The reabsorption process of urate in the kidney by the urate transporter URAT1 plays a pivotal role in controlling serum urate levels. URAT1 (SLC22A12) is a member of the SLC22 major facilitator superfamily transporters. The cryo-EM structures show that hURAT1 has the common architecture of SLC22 family transporters, which is formed by the N-terminal domain (NTD) with an extracellular protrusion and the C-terminal domain (CTD). Structural comparison between different conformations of hURAT1 reveals the rocker-switch-like mechanism for urate transport.

In the presence of substrate urate, hURAT1 predominantly adopts the outward-facing conformation, in which regions of the NTD and CTD in the inner leaflet of the plasma membrane bind to each other to seal the intracellular gate. Urate binds in the center of the transmembrane domain of hURAT1. The three protrusions on the electron density match the three oxygens on urate, unambiguously defining the binding pose of urate. The xanthine core of urate is wrapped by a hydrophobic cage consisting of five phenylalanines, including F241 of the NTD and F360, F364, F365, and F449 of the CTD. In addition to the binding by these five phenylalanines, the negatively charged 2’-oxygen of urate (pKa ~5.4)20 is coordinated by R477 on M11 and the 8’-OH of urate binds K393 on M8. In the outward-facing conformation, the lower regions of the NTD and CTD bind together to form the cytoplasmic gate below the urate-binding site. Particularly, F449 in the CTD blocks urate release through the cytoplasmic exit. On the cytosolic side of hURAT1, we found that E223 on M4 and R284 on H4 of the NTD made electrostatic interactions with R465 on M11 of the CTD and D525 on the loop between M12 and H7, respectively. To evaluate the functional importance of the observed polar interactions on the transporting activity of hURAT1, we mutated them into alanines to disrupt the interactions. We found that R465A and R284A mutants dramatically decreased the urate uptake activity of hURAT1, although with slightly decreased surface expression level, suggesting that both R465-E223 and R284-D525 interaction pairs play critical roles in stabilizing hURAT1 in the outward-facing conformation.

> GPEFMAFSELLDLVGGLGRFQVLQTMALMVSIMWLCTQSMLENFSAAVPSHRCWAPLLDNSTAQASILGSLSPEALLAISIPPGPNQRPHQCRRFRQPQWQLLDPNATATSWSEADTEPCVDGWVYDRSIFTSTIVAKWNLVCDSHALKPMAQSIYLAGILVGAAVCGPASDRFGRRLVLTWSYLQMAVSGTAAAFAPTFPVYCLFRFLLAFAVAGVMMNTGTLLMEWTSARARPLVMTLNSLGFSFGHGLTAAVAYGVRDWTLLQLAVSVPFFLCFLYSWWLAESARWLLTTGRLDRGLQELRRVAAINGKRAVQDTLTPEVLLSAMREELSVGQAPASLGTLLRTPGLRLRTCISTLCWFAFGFTFFGLALDLQALGSNIFLLQVLIGVVDIPAKMGALLLLSRLGRRPTLAASLLLAGLCILANTLVPHEMGALRSALAVLGLGGVGAAFTCITIYSSELFPTVLRMTAVGLGQMAARGGAILGPLVRLLGVHGPWLPLLVYGTVPVLSGLAALLLPETQSLPLPDTIQDVQNQAVKKATHGTLGNSVLKSTQF> DPTFYDIETLKVIDEEWQRTQCSPRETAVEVASELGKSTNTFFKPPCVNVFRCGGCCNEESLICMNTSTSYISKQLFEISVPLTSVPELVPVKVANHTGCKC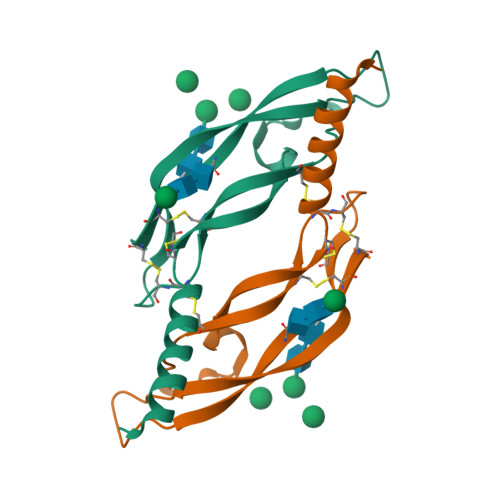LPTAHHHHHH> GEGLGGTFQKIPVALLTTTGRKTGQPRVNPLYFLRDGGRVIVAASKGGAEKNPMWYLNLKANPKVQVQIKKEVLDLTARDATDEERAEYWPQLVTMYPSYQDYQSWTDRTIPIVVC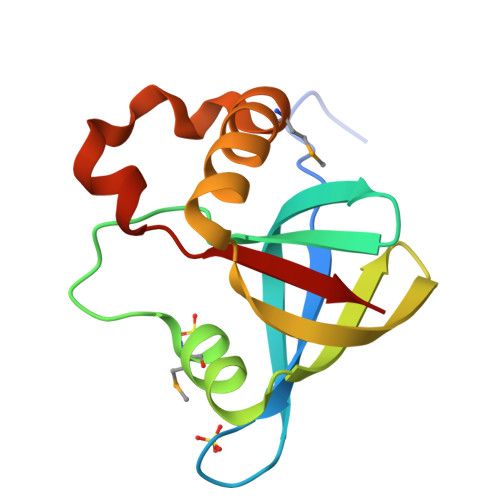EP> MSTPHHGRHELGQNFLSDRRVIADIVEIVSRTNGPIIEIGAGDGALTIPLQRLARPLTAVEVDARRARRLAQRTARSAPGPASRPTEVVAADFLRYPLPRSPHVVVGNLPFHLTTAILRRLLHGPGWTTAVLLMQWEVARRRAAVGGATMMTAQWWPWFEFGLARKVSAASFTPRPAVDAGLLTITRRSRPLVDVADRARYQALVHRVFTGR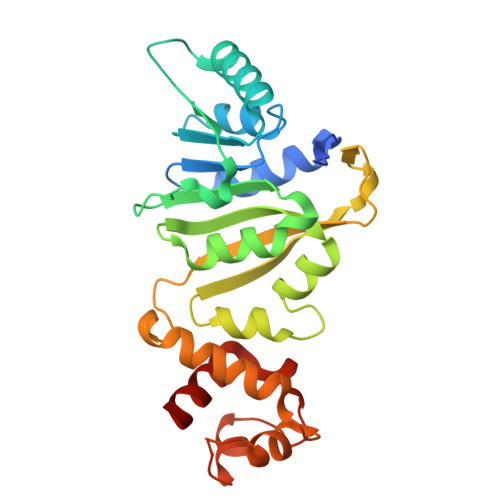GHGMAQILQRLPTPVPRTWLRANGIAPNSLPRQLSAAQWAALFEQTRLT>[2x]HMLPKDFQWGFATAAYQIEGAIDKDGRGPSIWDTFCAIPGKIADGTSGVTACDSYNRTAEDIALLKSLGAKSYRFSISWSRIIPKGGRDDPVNQLGIDHYAQFVDDLLEAGITPFITLFHWDLPEELHQRYGGLLNRTEFPLDFENYARVMFKALPKVRNWITFNEPWCSAILGYGSGTFAPGRQSTTEPWIVGHNLLVAHGRAVKVYRDEFKDLNDGQIGIVLNGDFTYPWDSSDPLDREAAERRLEFFTAWYADPIYLGDYPASMRKQLGDRLPEFTPEEKAFVLGSNDFYGMNHYTSNYIRHRTSPATADDTVGNVDVLFYNKEGQCIGPETESSWLRPCPAGFRDFLVWISKRYNYPKIYVTENGTSLKGENDLPKEKILEDDFRVNYYNEYIRAMFTAATLDGVNVKGYFAWSLMDNFEWADGYVTRFGVTYVDYENGQQRFPKKSAKSLKPLFDELIAKE

Our laboratory has previously reported the crystal structure and biochemical characterisation of a glycoside hydrolase family 1 (GH1) β-glucosidase highly expressed by Trichoderma harzianum (ThBgl) under biomass degradation conditions. β-glucosidase (EC 3.2.1.21) catalyses the hydrolysis of β-glucosidic linkages in aryl-, amino-, or alkyl-β-D-glucosides and di- or oligosaccharides at the nonreducing ends, releasing β-D-glucose monomers. This class of enzymes has a critical role within the set of enzymes that compose the enzymatic cocktails designed for plant biomass hydrolysis, thereby alleviating the inhibition of other cellulases by cellobiose during the reaction. ThBgl is easily inhibited by glucose. The molecular basis of glucose tolerance in β-glucosidases is not completely known; however, it has been correlated with structural features at the entrance channel to the active site rather than the active site itself.

The tailored ThBgl (ThBgl-Mut) crystal structure revealed that the selected mutations mimicked the active-site entrance of the highly glucose-tolerant GH1 β-glucosidase from Humicola insolens (HiBG), acting as gatekeepers, as postulated for the HiBG glucose tolerance mechanism. As expected, the mutations did not affect the overall tertiary structure, thereby preserving the conserved GH1 (α/β)8-TIM barrel fold. The ThBgl-Mut and ThBgl-WT structures are very similar and display a r.m.s.d. value of 0.28 Å over 464 Cα atoms, with each monomer being considered. Moreover, the predicted catalytic residues E165 (acid–base) and E366 (nucleophile) are spatially conserved and thus not affected by the rational modifications. As predicted by our structural analysis, the mutated residues W167 and L172 function as gatekeepers and affect the positive-subsite region topology, narrowing the ThBgl active-site pocket, while the −1 subsite is fully conserved. At the other extremities of these residues, the conserved W338 (corresponding to the residues W349 in HiBgl and W339 in TrBgl) delineates the new, narrowed entrance to the active site. The L167W/P172L double mutation had a significant impact on the glucose tolerance and stimulation of ThBgl. In the presence of 0.1–0.25M glucose, although ThBgl-WT showed an accelerated decline in activity, ThBgl-Mut reached its highest levels, which represented an approximately 300% increase over the value measured under the no glucose conditions. In fact, the catalytic efficiency parameter (kcat/KM) of ThBgl-Mut is approximately 5-fold higher than that of ThBgl-WT under the conditions assayed.> MAGETDLQKILRESNDQFTAQMFSEVVKANPGQNVVLSAFSVLPPLGQLALASVGESHDELLRALALPNDNVTKDVFADLNRGVRAVKGVDLKMASKIYVAKGLELNDDFAAVSRDVFGSEVQNVDFVKSVEAAGAINKWVEDQTNNRIKNLVDPDALDETTRSVLVNAIYFKGSWKDKFN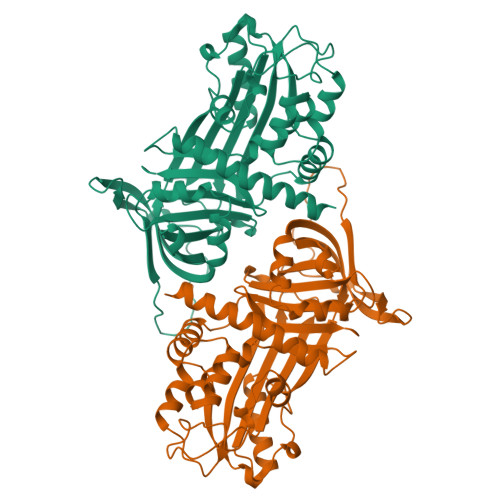KERTMDRDFHVSKDKTIKVPTMIGKKDVRYADVPELDAKMIEMSYEGDQASMIIILPNQVDGITALEQKLKDPKALSRAEERLYNTEVEIYLPKFKIETTTDLKEVLSNMNIKKLFTPGAARLENLLKTKESLYVDAAIQKAFIEVNEEGAEAAAANAFKITTYSFHFVPKVEINKPFFFSLKYNRNSMFSGVCVQP>[8x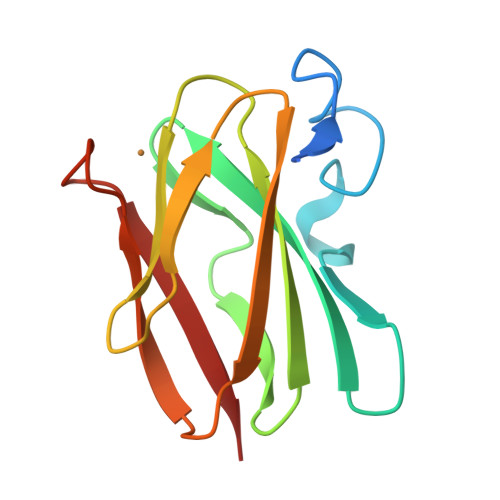]GSHMVIPAGKLERVDPTTVRQEGPWADPAQAVVQTGPNQYTVYVLAFAFGYQPNPIEVPQGAEIVFKITSPDVIHGFHVEGTNINVEVLPGEVSTVRYTFKRPGEYRIICTPHPFMFGTIVVKE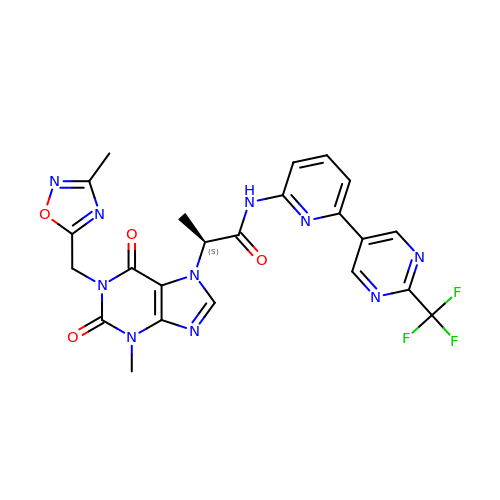(2S)-2-{3-methyl-1-[(3-methyl-1,2,4-oxadiazol-5-yl)methyl]-2,6-dioxo-1,2,3,6-tetrahydro-7H-purin-7-yl}-N-{6-[2-(trifluoromethyl)pyrimidin-5-yl]pyridin-2-yl}propanamide | C23 H19 F3 N10 O4 | UMRMICUACMEDEJ-UHFFFAOYSA-N> GSHMETSK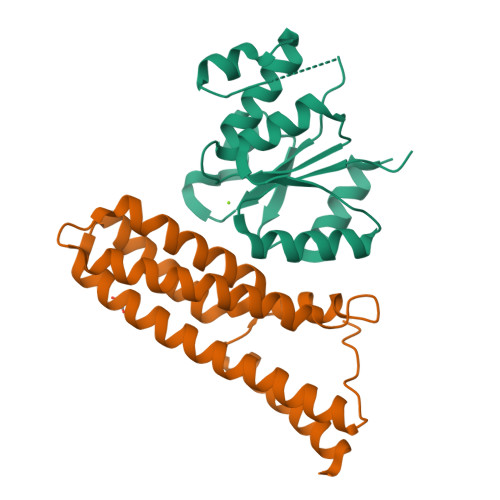PKILLVEDNKINIMVAKSMMKQLGHTMDIANNGVEAITAINSSSYDLVLMDVCMPVLDGLKATRLIRSYEETGNWNAAIEAGVDISTSENEQVCMRPTNRLPIIAMTANTLAESSEECYANGMDSFISKPVTLQKLRECLQQYLH;> GPLGSMDLVQKQKSLQDYTKSLFLEGILDSQFLQLQQLQDESNPDFVSQVVTLFFQDSDRILNDLSLSLDQQVVDFKKVDPHVHQLKGSSSSIGAQRVKNACVVFRSFCEQQNVEACHRCLQQVKQEYYLVKNRLETLFKLEQQIVASGGMIPAVELGF>[2x]PF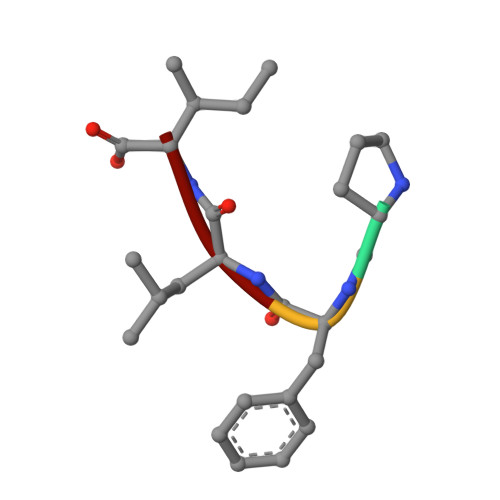LI> MGSSHHHHHHENLYFQGSMEQAIINDEREYLRHFWHPVCTVTELEKAHPSSLGPLAVKLLNEQLVVAKLGDEYVAMRDRCAHRSAKLSLGTVSGNRLQCPYHGWQYDTHGACQLVPACPNSPIPNKAKVDRFDCEERYGLIWIRLDSSFDCTEIPYFSAANDPRLRIVIQEPYWWDATAERRWENFTDFSHFAFIHPGTLFDPNNAEPPIVPMDRFNGQFRFVYDTPEDMAVPNQAPIGSFSYTCSMPFAINLEVSKYSSSSLHVLFNVSCPVDSHTTKNFLIFAREQSDDSDYLHIAFNDL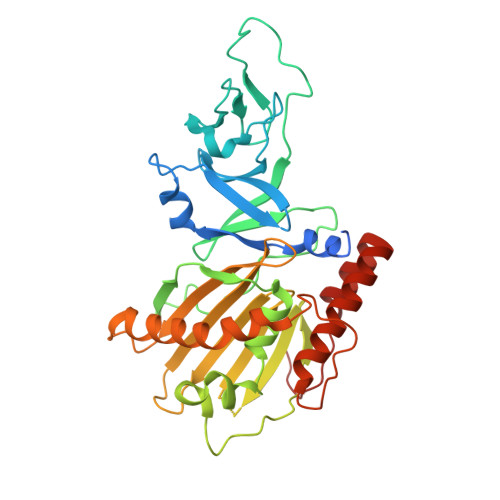VFAEDKPVIESQWPKDAPADEVSVVADKVSIQYRKWLRELKEAHKEGSQAFRSALLDPVIESDRSYI> MQSGSRPHLAWQREHMWLALQGLGFESGAEAANAGKTLVHVTFGVNMFDKPNKDAFYVVFHFLFGKLDNVRCKEVFRYCWPPLDKKRDAEFRKACCEWLKKISDEVGAGFPQVVASIFLSPGGPKFVHLLYHFARYVMLQHIKRDADAGNVFISEALQSKIQDPQKALARNKLARQKYLKVLQKENLVIEEYQRKAQLLIKQIRDMRSEHVALQNQQKLAEKVDRKISDKDENIQKTRCMWNTIMQMLKEMEKEVDVVDAVVRGNIDQYCLDGTNATLNIPNLLISRIESEMHRLQMDNVYEAGKVNLITVVQLLNEALKLVSGERSLYDCKGVRLDLQYLHGKAKFESEVLTRLRNMRHKIKREDLVSIEKIIADREREWERKWEKILGKCPFSLLKGLNPALELNPPMAPFSFDPASEEVLKSSVFCHYPASLQEYSHKEKPLKDFNQDHSGELVQRLIGATVLTRSGRKSTSSLGMATPNRRRMSLNEREFQTPTMNDRIGFQRTPSSAVQKRRADVSWKTAANSPLPCTPTPYKQDPKNMARQQLAQQVADYIVSESPRSSGGRGMELDDLLGVLSSDPFLSRKEIPRTPENLISDIRSSWRKAIQSEESLVVASPVAAPCMDSTAELESAHCSQIDLSMACFLSTSHASDQNDCSGTRIPHNTGGNKASSLHSDVVHHESIDMKSEIDSSQPEDLSLPIKENEPADKLINLLDDKKESENADTLTNPVEFIFSNQPISKLMDKTMFISVSGQENLSAHTTLSWNSSNMITSDSSSDTHEIIQFGILHETLPENAGNVSLNSTLSLGGNEEPFEKSELSDHDFTFDRKEHSSRSMEGKMDINSIRSRYEALKRTLTSLTDEEYHGDPDTSNMRFTKHKSESSLILGSDV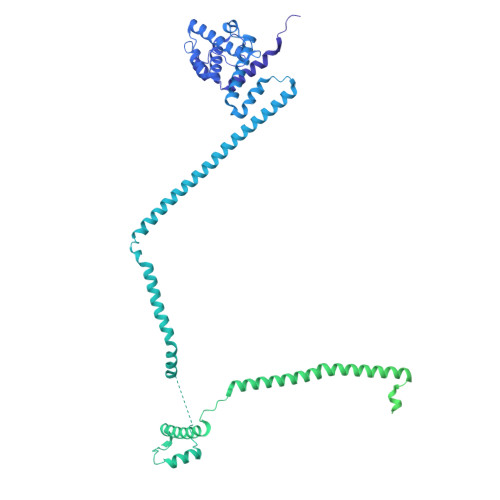YSPVEKVLSLDLEYLTTPSPKDRKLSLPQLISFSPETIRSEKQEDLLDVFESQDFVNPNKTFDFTSSGLDLQKSTDEGPEQLIKL Nucleotide-sugar transporters (NSTs) transport nucleotide-sugar conjugates into the Golgi lumen where they are then used in the synthesis of glycans. The CMP-sialic acid transporter (CST) is one of seven types of mammalian NSTs and is highly selective for transporting CMP-sialic acid (CMP-Sia) into the Golgi lumen as well as for transporting the free nucleotide byproduct of the glycosyltransferase reaction, CMP, back to the cytoplasm. Here, we describe the discovery that an endogenous methylated form of cytidine monophosphate (m5CMP) binds and inhibits CST. The presence of m5CMP in cells results from the degradation of RNA that has had its cytosine bases post-transcriptionally methylated through epigenetic processes.

In order to understand the molecular details of how m5CMP binds CST with a higher affinity than CMP, we determined the X-ray crystal structure of CST in complex with m5CMP. Crystals of CST were grown using the lipidic cubic phase method, in the presence of 400 μM m5CMP. However, one key difference is that the CST-m5CMP crystals diffracted X-rays to a much higher resolution of 1.8 Å (compared to 2.6 Å for the CST-CMP crystals). This let us build a highly-detailed model which contained 13 lipid molecules and 162 waters resulting in a Rwork and Rfree of 18.5% and 19.8%, respectively. Overall, the CST-m5CMP structure is very similar to the CST-CMP structure, with a r.m.s.d. of 0.17 Å. m5CMP binds in an essentially identical orientation as CMP does and there are no obviously-significant differences in the conformation of the residues that line the substrate-binding cavity. The eponymous methyl group of m5CMP occupies a small and mostly-hydrophobic pocket. This pocket is present but vacant in the CMP-bound structure which explains how CST can accommodate the addition of a methyl group at the C-5 position on the pyrimidine ring. By comparing the two structures, it seems that the burial of m5CMP’s C-5 methyl in this hydrophobic pocket is the primary contributor to the 16-fold increase in m5CMP’s binding affinity compared to CMP, on account of the hydrophobic effect. The residues that line the methyl-interacting hydrophobic pocket–primarily Phe195, Thr260 (Cγ2 atom), and Val264, but also Tyr98, Gly192, Met213, and Ser261 (only Cα and Cβ atoms) are highly conserved among orthologous CST proteins (SLC35A1 gene products) from other organisms, suggesting that the ability for CST to bind m5CMP is a conserved property across species. However, including increasing amounts of m5CMP during the 41°C incubation leads to more and more protein being protected from denaturation, to the point where saturating amounts of m5CMP are able to prevent any denaturation–as indicated by the peak height for the 100 μM sample being identical to the sample that was kept at 4°C. By plotting peak heights against ligand concentration, we can determine an apparent Kd of 1.0 ± 0.1 μM.

> MAPARENVSLFFKLYCLTVMTLVAAAYTVALRYTRTTAEELYFSTTAVCITEVIKLLISVGLLAKETGSLGRFKASLSENVLGSPKELAKLSVPSLVYAVQNNMAFLALSNLDAAVYQVTYQLKIPCTALCTVLMLNRTLSKLQWISVFMLCGGVTLVQWKPAQATKVVVAQNPLLGFGAIAIAVLCSGFAGVYFEKVLKSSDTSLWVRNIQMYLSGIVVTLAGTYLSDGAEIQEKGFFYGYTYYVWFVIFLASVGGLYTSVVVKYTDNIMKGFSAAAAIVLSTIASVLLFGLQITLSFALGALLVCVSIYLYGLPRQDTTSNSLEVLFQ>MGGHHHHHHGLEVLFQGPQEKDASSQGFLPHFQHFATQAIHVGQDPEQWTSRAVVPPISLSTTFKQGAPGQHSGFNYSRSGNPTRNCLEKAVAALDGAKYCLAFASGLAATVTITHLLKAGDQIICMDDVYGGTNLYFRQVASEFGLKISFVDCSKIKLLEAAITPETKLVWIETPTNPTQKVIDIEGCAHIVHKHGDIILVVDNTFMSPYFQRPLALGADISMYSATKYMNGHSDVVMGLVSVNCESLHNRLRFLQNSLGAVPSPIDCYLCNRGLKTLHVRMEKHFKNGMAVAQFLESNPWVEKVIYPGLPSHPQHELVKRQCTGCTGMVTFYIKGTLQHAEIFLKNLKLFTLAVSLGGFESLAELPAIMTHASVLKNDRDVLGISDTLIRLSVGLEDEEDL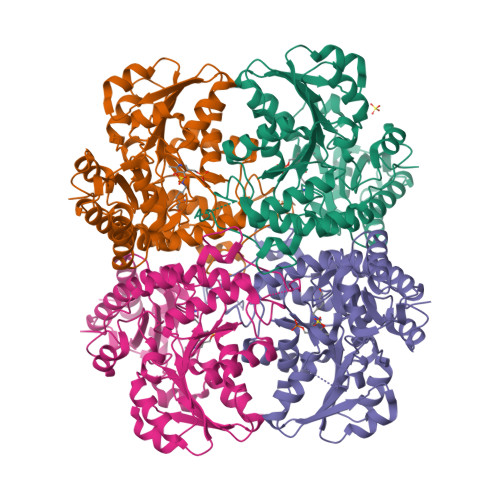LEDLDQALKAAHPPSGSHS[8x]>MTTLTRADWEQRAQNLKIEGRAFIQGEYTAAASGETFDCISPVDGRLLAKVASCDAADAQRAVESARSAFDSGAWSRLAPAKRKATMIRFAGLLEQNAEELALLETLDMGKPISDSLGVDIPGGARALSWSGEAIDKLYDEVAATPHDQLGLVTREPVGVVAAIVPWNFPLMMACWKLGPALSTGNSVVLKPSEKSPLTAIRIAQLAIEAGIPAGVLNVLPGYGHTVGKALALHMDVDTVVFTGSTKIAKQLMIYAGESNMKRVWLEAGGKSPNIVFADAPDLQAAADSAASAIAFNQGEVCTAGSRLLVERSIKDRFLPMVIEALGTWKPGNPLDPATNVGALVDTQQMNTV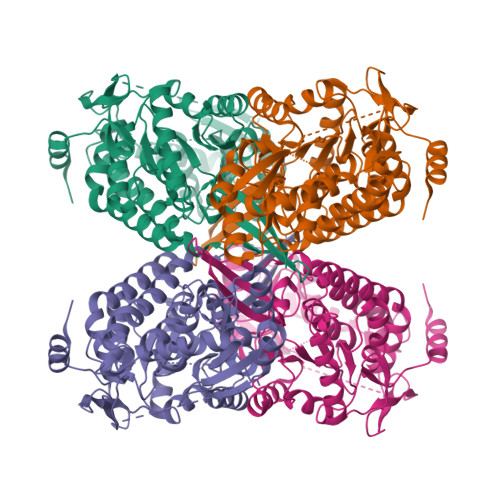LSYIAAGHTDGARLVAGGKQILQETGGTYVEPTIFDGVNNAMRIAQEEIFGPVLSVLTFDTAEEAIQIANDTPYGLAAAVWTANLSKAHLTARALRAGSVWVNQYDGGDMTAPFGGFKQSGNGRDKSLHAFDKYTELKSTWIKL[2x]>MDFPQQLEACVKQANQALSRFIAPLPFQNTPVVETMQYGALLGGKRLRPFLVYATGHMFGVSTNTLDAPAAAVECIHAYSLIHDDLPAMDDDDLRRGLPTCHVKFGEANAILAGDALQTLAF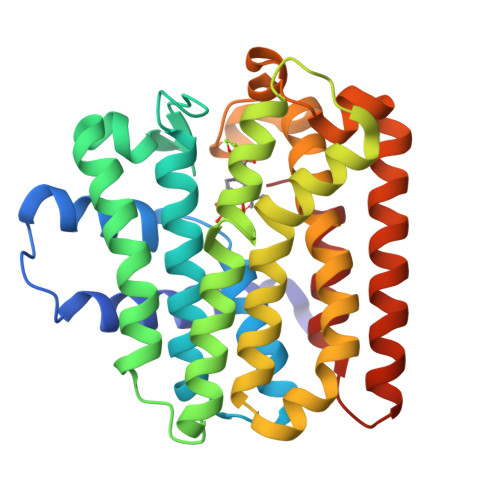SILSDADMPEVSDRDRISMISELASASGIAGMCGGQALDLDAEGKHVPLDALERIHRHKTGALIRAAVRLGALSAGDKGRRALPVLDKYAESIGLAFQVQDDILDVVGDTATLGKRQGADQQLGKSTYPALLGLEQARKKARDLIDDARQSLKQLAEQSLDTSALEALADYIIQRNK[2x]> XVALDPIDISIVLNKIKSDLEESKEWIRRSNQKLDS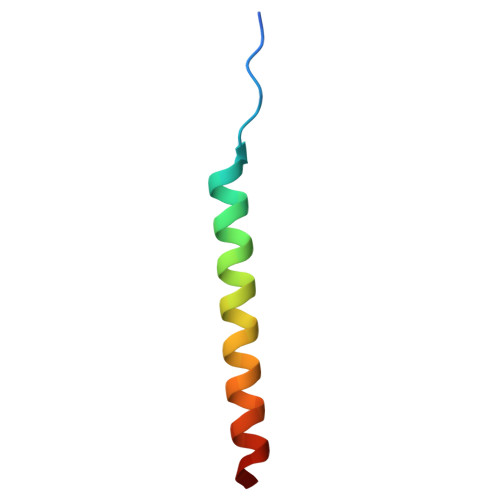IX> PTPSSTPSVLGEYGQRFMWLWNKIHDPANGYFNQDGIPYHSVETLICEAPDYGHLTTSEAFSYYVWLEAVYGKLTGDWSKFKTAWDTLEKYMIPSAEDQPMRSYDPNKPATYAGEWETPDKYPSPLEFNVPVGKDPLHNELVSTYGSTLMYGMHWLMDVDNWYGYGKRGDGVSRASFINTFQRGPEESVWETVPHPSWEEFKWGGPNGFLDLFIKDQNYSKQWRYTDAPDADARAIQATYWAKVWAKEQGKFNEISSYVAKAAKMGDYLRYAMFDKYFKPLGCQDKNAAGGTGYDSAHYLLSWYYAWGGALDGAWSWKIGSSHVHFGYQNPMAAWALANDSDMKPKSPNGASDWAKSLKRQIEFYRWLQSAEGAIAGGATNSWNGRYEKYPAGTATFYGMAYEPNPVYHDPGSNTWFGFQAWSMQRVAEYYYVTGDKDAGALLEKWVSWVKSVVKLNSDGTFAIPSTLDWSGQPDTWNGAYTGNSNLHVKVVDYGTDLGITASLANALLYYSAGTKKYGVFDEGAKNLAKELLDRMWKLYRDEKGLSAPEKRADYKRFFEQEVYIPAGWIGKMPNGDVIKSGVKFIDIRSKYKQDPDWPKLEAAYKSGQAPEFRYHRFWAQCDIAIANATYEILFGNQSSSVDKLAAALE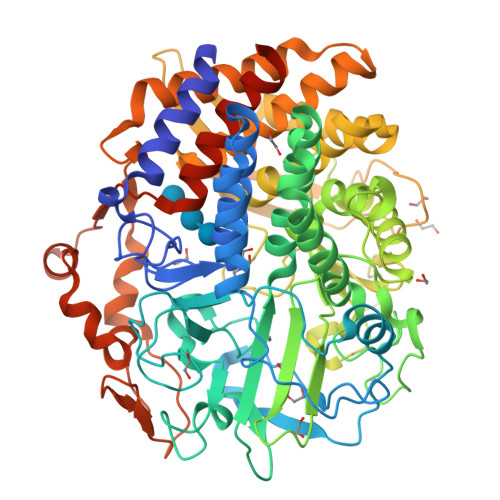HHHHHH>MHHHHHHENLYFQGMNDEPRWLTAEEQLVWRSYIEAATLLEDHLDRQLQRDAGMPHVYYGLLVKLAESPRRRLRMTELAKYAKITRSRLSHAVARLEKNGWVRREDCPSDKRGQFAILTDEGYEVLRRTAPGHVDAVRQAVFDRLTPEQQKSLGEIMRIVAEGLQPSEAGADLPWLR[4x]

MarR family transcriptional regulators (MFRs) are widespread across bacteria and archaea, where they regulate various functions, including the response to oxidative stress (1–3), pathogenesis and antibiotic resistance, and are thus of significant clinical interest. MFRs are one-component response regulators, having input and output domains fused in a single protein chain. They function as homodimers and regulate gene expression by binding to pseudopalindromic DNA sequences through winged-helix DNA-binding motifs. Most MFRs are repressors, and their abilities to bind DNA are abrogated by the binding of small molecule ligands or by sensing reactive oxygen species via reactive cysteine residues. Using this approach, we identified two potential operator sites upstream of sco3205, which encodes a putative MFR, one of 42 in the Streptomyces coelicolor genome.

Guided by the operator sequences, we determined through SPR footprinting, we go on to crystallize and solve the X-ray structure of a SCO3205-DNA complex at 2.8 Å resolution. The resultant crystal structure reveals two SCO3205 homodimers in the ASU, each bound to its own ds 22-mer DNA. The SCO3205 homodimers are closely similar (root mean square deviation based on Cα atoms = 0.16 Å) and adopt the typical MFR overall triangular shape. The DNA-binding domain contains helices α2, α3 and α4 and the β-sheet and includes a winged helix DNA-binding motif, where α3 and α4 form a classical helix-turn-helix, and the loop delineated by β2 and β3 corresponds to the ‘wing’. The SCO3205 dimer makes extensive contacts with the DNA duplex spanning some 1920 Å2 (calculated using PISA), and the majority of the interactions fall into three types. Those involving the helix-turn-helix motif, those involving the wing, and those involving the C-terminal tail. The recognition helices (α4 and α4′) engage with consecutive major grooves and interact with both the bases and the phosphate backbone. Contacts with DNA bases in the major groove are made by just three residues: Arg72, Ser73 and His77. Perhaps, the most significant interactions involve Arg98: the electropositive guanidinium group is inserted into the minor groove, where the electronegative potential of the phosphate backbone is focused, and it donates hydrogen bonds to both the O4' of the deoxyribose moiety and N3 of A3 via its Nη2 and Nε atoms, respectively. The C-terminal residue itself, Arg163, has a dual function: the side-chain anchors the tail to the core of the homodimer via salt bridges to Asp28 in helix α1, whereas via a further salt bridge, the carboxy terminus orients the guanidinium group of Arg72 (in the recognition helix) for interaction with either N7 of A5, or the phosphate group of G4.>MRLTILGMTAHDSRPEQAKKLADIDWSTLGFSYIRTDLRYLAHWKDGEWDAGTLTEDNQIHLAEGSTALHYGQQCFEGLKAYRCADGSINLFRPDQNAARMRMSCRRLLMPELSDEQFIDACLQVVRANEHFLPPYGTGGSLYLRPFVIGVGDNIGVRTAPEFIFSVFCVPVGPYFKGGLTPTNFITSDYDRAAPH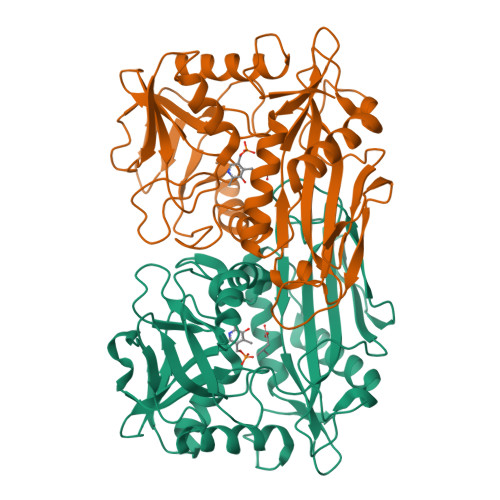GTGAAKVGGNYAASLLPGYEAKKRDFADVIYLDPATHTTIEEAGAANFFAITQDGQKFVTPQSPSILPSITKYSLLWLAEHRLGLEVEEGDIRIDELGKFSEAGACGTAAVITPIGGIQHGDDFHVFYSESEPGPVTRRLYDELVGIQYGDKEAPEGWIVKV[4x]> MQDPDGIDINTKIFNSVAEVFQKAQGSYAGHRKHIAVLKKIQSKAVEQGYEDAFNFWFDKLVTKILPLKKNEIIGDRIVKLVAAFIASLERELILAKKQNYKLTNDEEGIFSRFVDQFIRHVLRGVESPDKNVRFRVLQLLAVIMDNIGEIDESLFNLLILSLNKRIYDREPTVRIQAVFCLTKFQDEEQTEHLTELSDNEENFEATRTLVASIQNDPSAEVRRAAMLNLINDNNTRPYILERARDVNIVNRRLVYSRILKSMGRKCFDDIEPHIFDQLIEWGLEDRELSVRNACKRLIAHDWLNALDGDLIELLEKLDVSRSSVCVKAIEALFQSRPDILSKIKFPESIWKDFTVEIAFLFRAIYLYCLDNNITEMLEENFPEASKLSEHLNHYILLRYHHNDISNDSQSHFDYNTLEFIIEQLSIAAERYDYSDEVGRRSMLTVVRNMLALTTLSEPLIKIGIRVMKSLSINEKDFVTMAIEIINDIRDDDIEKQEQEEKIKSKKINRRNETSVDEEDENGTHNDEVNEDEEDDNISSFHSAVENLVQGNGNVSESDIINNLPPEKEASSATIVLCLTRSSYMLELVNTPLTENILIASLMDTLITPA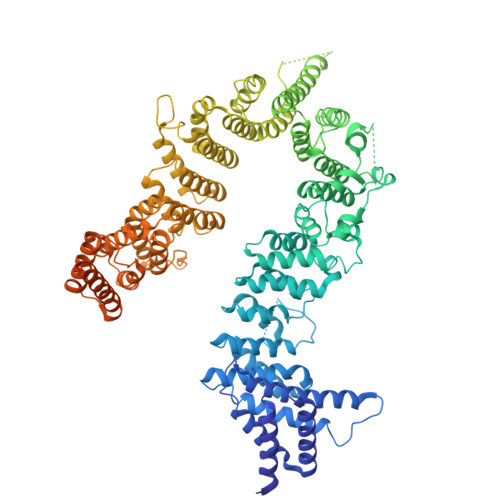VRNTAPNIRELGVKNLGLCCLLDVKLAIDNMYILGMCVSKGNASLKYIALQVIVDIFSVHGNTVVDGEGKVDSISLHKIFYKVLKNNGLPECQVIAAEGLCKLFLADVFTDDDLFETLVLSYFSPINSSNEALVQAFAFCIPVYCFSHPAHQQRMSRTAADILLRLCVLWDDLQSSVIPEVDREAMLKPNIIFQQLLFWTDPRNLVNQTGSTKKDTVQLTFLIDVLKIYAQIEKKEIKKMIITNINAIFLSSEQDYSTLKELLEYSDDIAENDNLDNVSKNALDKLRNNLNSLIEEINERSETQTKDENNTANDQYSSILGNSFNKSSNDTIEHAADITDGNNTELTKTTVNISAVDNTTEQSNSRKRTRSEAEQIDTSKNLENMSIQDTSTVAKNVSFVLPDEKSDAMSIDEEDKDSESFSEVC>[4x]MAHHHHHHSSGLEVLFQGPMTERLETRPQALLI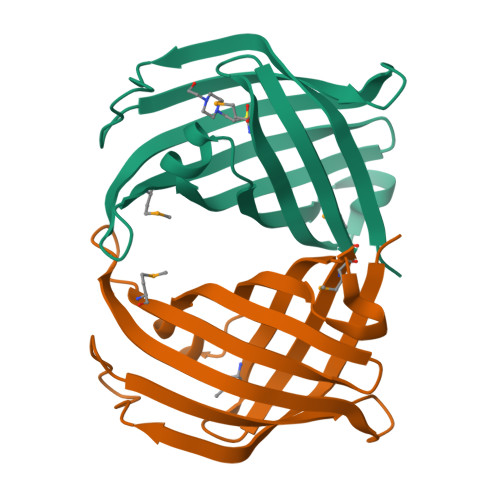KVPTEIVVKVVDDVDVAAPAVGQVGKFDDELYDEAGAQIGTSSGNFRIEYVRPTDGGLMTYYQEDITLSDGVIHAEGWADFNDVRTSKWVFYPATGVSGRYLGLTGFRQWRMTGVRKSAEARILMGE>[10x]MLVSVYLALLVACVGQAHSQANLMRLKSDLFNRSPMYPGPTKDDPLTVTLGFTLQDIVKVDSSTNEVDLVYYEQQRWKLNSLMWDPNEYGNITDFRTSAADIWTPDITAYSSTRPV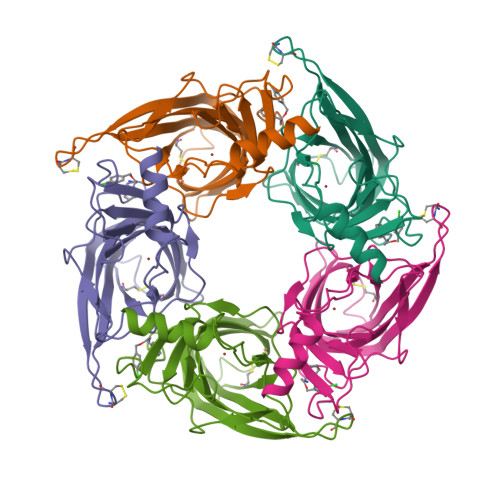QVLSPQIAVVTHDGSVMFIPAQRLSFMCDPTGVDSEEGVTCAVKFGSWVYSGFEIDLKTDTDQVDLSSYYASSKYEILSATQTRQVQHYSCCPEPYIDVNLVVKFRERRAGNGFFRNLFD>[2x]MAHHHHHHMTQAFTVVIPARYASTRLPGKPLQDIAGQPMIQRVWNQARKSAASRVVVATDDERILAACQGFGAEALLTRAEHNSGTDRLEEVASRLGLASDAIVVNVQGDEPLIPPALIDQVAANLAAHPEAAIATLAEPIHEVSALFNPNVVKVATDIDGLALTFSRAPLPWARDAFARDRDSLPEGVPYRRHIGIYAYRVGFLADFVAWGPCWLENAESLEQLRA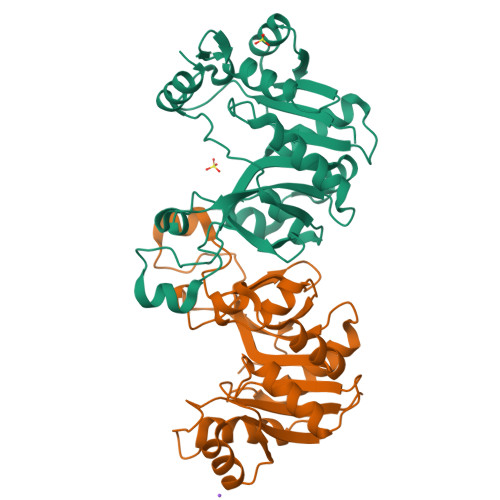LWHGVRIHVADARENMLPGVDTPEDLERVRRVLGG>[2x]ADFEVHMLNKGKDGALVFEPASLKVAPGDTVTFIPTDKGHNVETIKGMIPDGAEAFKSKINENYKVTFTAPGVYGVKCTPHYGMGMVGVVQVGDAPANLEAVKGA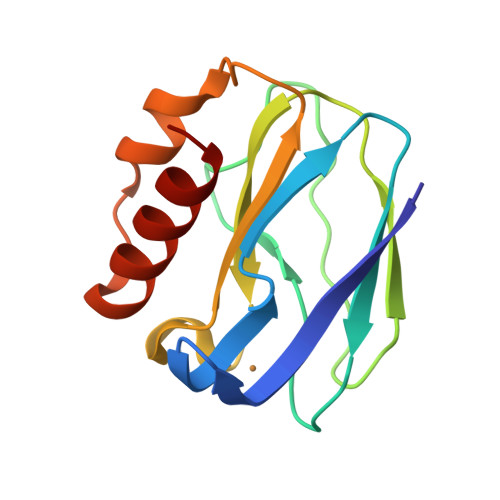KNPKKAQERLDAALAALGN1-(3-deoxy-3-fluoro-beta-D-glucopyranosyl)-5-fluoropyrimidine-2,4(1H,3H)-dione 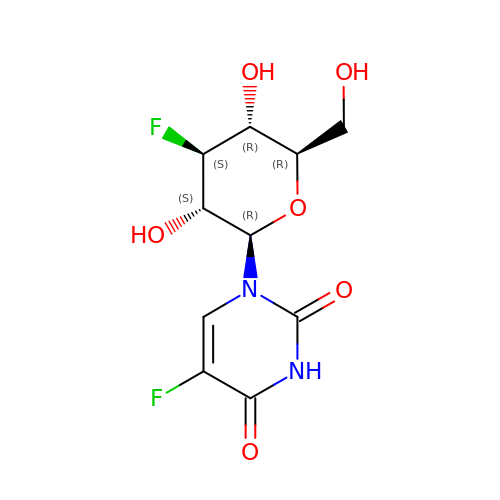| C10 H12 F2 N2 O6 | BXHWKGLMPCAUQA-XLKNOJSPSA-N> MVSLFKRGKAPPLTKEGPTSKKPP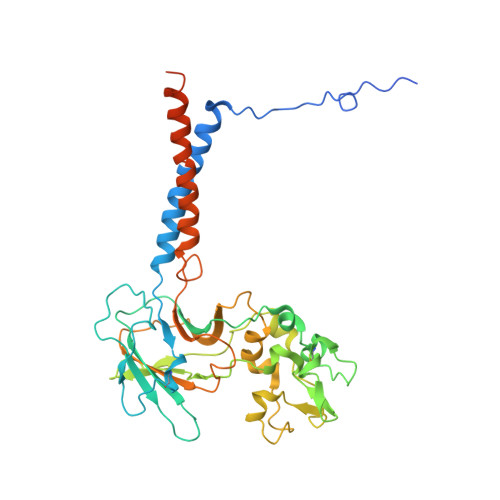NTAFRQQRLKAWQPILSPQSVLPLLIFVACIFTPIGIGLIVSATKVQDLTIDYSHCDTKASTTAFEDIPKKYIKYHFKSKVENKPQWRLTENENGEQSCELQFEIPNDIKKSIFIYYKITNFYQNHRRYVQSFDTKQILGEPIKKDDLDTSCSPIRSREDKIIYPCGLIANSMFNDTFSQVLSGIDDTEDYNLTNKHISWSIDRHRFKTTKYNASDIVPPPNWMKKYPDGYTDENLPDIHTWEEFQVWMRTAAFPKFYKLTLKNESASLPKGKYQMNIELNYPISLFGGTKSFVLTTNGAIGGRNMSLGVLYLIVAGLCALFGIIFLVKLIFQPRAMGDHTYLNFDDEENEDYEDVHAENTTLREIL> DILTVEKLYRPSHEYGFLRETDTVKD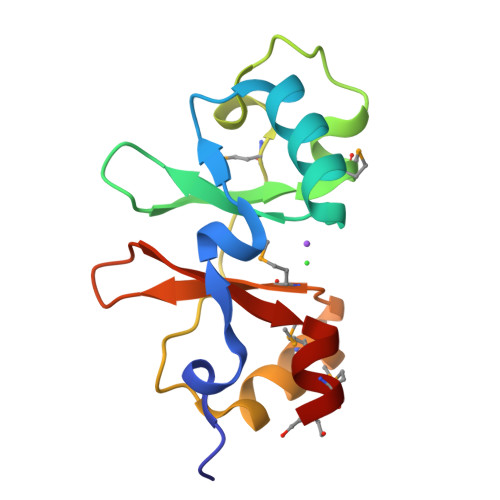YLDLVRKNRSSRFPVINQHQVVVGVVTMRDAGDKSPSTTIDKVMSRSLFLVGLSTNIANVSQRMIAEDFEMVPVVRSNQTLLGVVTRRDVMEK> GAMAEEQMRLPSADVYRFAEPDSEENIIFEENMQPKAGIPIIKAGTVIKLIERLTYHMYADPNFVRTFLTTYRSFCKPQELLSLIIERFEIPEPEPTEADRIAIENGDQPLSAELKRFRKEYIQPVQLRVLNVCRHWVEHHFYDFERDAYLLQRMEEFIGTVRGKAMKKWVESITKIIQRKKIARDNGPGHNITFQSSPPTVEWHISRPGHIETFDLLTLHPIEIARQLTLLESDLYRAVQPSELVGSVWTKEDKEINSPNLLKMIRHTTNLTLWFEKCIVETENLEERVAVVSRIIEILQVFQELNNFNGVLEVVSAMNSSPVYRLDHTFEQIPSRQKKILEEAHELSEDHYKKYLAKLRSINPPCVPFFGIYLTNILKTEEGNPEVLKRHGKELINFSKRRKVAEITGEIQQYQNQPYCLRVESDIKRFFENLNPMGNSMEKEFTDYLFNKSLEIEPRNPKPLPRFPKKYSYPLKSPGVRPSNPRPGTMRHPTPLQQEPRKISYSRIPESETESTASAPNSPRTPLTPPPASGASSTTDVCSVFDSDHSSPFHSSNDT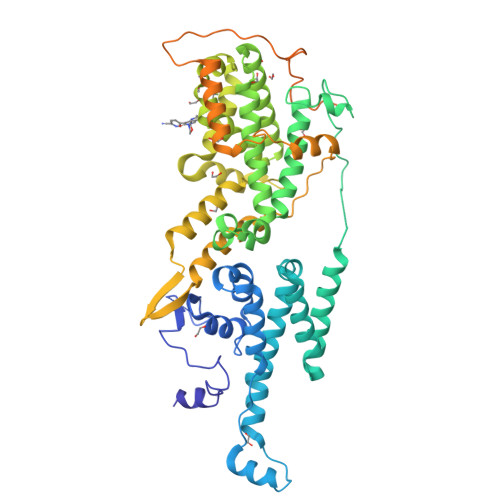VFIQVTLPHGPRSASVSSISLTKGTDEVPV> GGAGGGAAAAGUUAUCAGGCAUGCACCUGGUAGCUAGUCUUUAAACCAAUAGAUUGCAUCGGUUUAAAAGGCAAGACCGUCAAAUUGCGGGAAAGGGGUCAACAGCCGUUCAGUACCAAGUCUCAGGGGAAACUUUGAGAUGGCCUUGCAAAGGGUAUGGUAAUAAGCUGACGGACAUGGUCCUAACCACGCAGCCAAGUCCUAAGUCAACAGAUCUUCUGUUGAUAUGGAU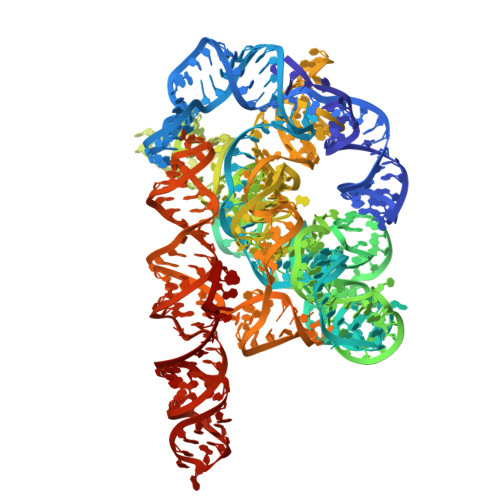GCAGUUCACAGACUAAAUGUCGGUCGGGGAAGAUGUAUUCUUCUCAUAAGAUAUAGUCGGACCUCUCCUUAAUGGGAGCUAGCGGAUGAAGUGAUGCAACACUGGAGCCGCUGGGAACUAAUUUGUAUGCGAAAGUAUAUUGAUUAGUUUUGGAG>[4x]AGFSMDKANSEACRDG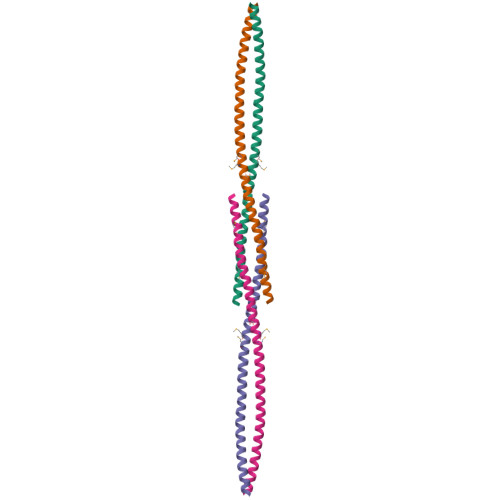LRAVMECRNVTHLLQQELTEAQKGFQDVEAQAATCNHTVMALMASLDAEKAQGQKKVEELEGEITTLNHKLQDASAEVERLRRENQVLSVRIADKKYYPSSQDSS The multi-subunit Type III-A CRISPR-Cas effector complex (Csm) exemplifies this principle and is in addition regulated by cellular metabolites such as divalent metals and ATP. Recognition of the foreign or cognate target RNA (CTR) triggers its single-stranded deoxyribonuclease (DNase) and cyclic oligoadenylate (cOA) synthesis activities. The same activities remain dormant in the presence of the self or non-cognate target RNA (NTR) that differs from CTR only in its 3′-protospacer flanking sequence (3′-PFS). The single-stranded DNase (ssDNase) and the cOA synthesis activities reside within the Csm1 subunit and the RNase activity resides within Csm317–19.

In contrast, a target RNA that complements both the guide region and the 5′-tag of the crRNA (alternatively referred to as the non-cognate target RNA, or NTR) is unable to switch on the Csm1-mediated activities. The 3′-PFS of NTR differs from that of CTR-43 and bears a complementary sequence to that of the crRNA 5′ tag. Seven of the eight PFS nucleotides are observed and only four form base pairs with the 5′ tag. Nucleotide (-1)′ is flipped out by the thumb loop of Csm4 similar to those at the cleavage sites. Nucleotides (-2)′–(-5)′ base pair with nucleotides (2–5) of the 5′ tag and (-6)′–(-7)′ rest on a groove formed by the Lid loop of Csm4 and the LiP loop of LlCsm1. Though the Csm1-Csm4 interface further reduces from 1261 Å2 in the CTR-bound to 929 Å2 in the NTR-bound complex, LlCsm1 gains 433 Å2 interfaces with 3′-PFS that in turn bases pairs with the 5′ tag of crRNA. As a result, 3′-PFS establishes an extensive interface that stabilizes Csm1 onto Csm4 and crRNA. Given the close resemblance in Csm1 structure between the CTR- and the NTR-bound LlCsm and the large distance between the 3′-PFS binding site and the HD domain, the strikingly different enzymatic activities between the two may be accounted for by their different dynamic behaviors. The refined atomic displacement parameter, or the B factor, combined with the map-fitting quality score, Q score, provides an indication that the Csm1 subunit is less stable in the CTR- than in the NTR-bound complex.

> MDKINLVCGSLLHNIGKIIYRGTSERAKHSKLGGDFIKSFEQFRNTELTDCIRYHHAQEITSVKSNKEKNSLFYITYIADNISSGMDRRKDLEEGAEGFNWDKKVALGSVFNVLNEKEKGRQNYSYPFVARTRIKEEPLNFPTATQNQYTTSYYDGLITDMKTILQRLKPDKEHINSLLQMMESLWSYVPSSTDKNQLVDISLYDHSRTTAAIASAIYDYFQAENITDYQKELFDYNATEFYDKNAFLMMNFDMSGVQNFIYNISGSKALKSLRARSFYLDMLLEYISDNLLEKLELSRANILYVGGGHAYLLLANTNKTKAILSDFEHDLKTWFLDKFKIDLYVAMAYTEVSANDLMNHNGHYRDIYRRLSQKTSAKKANRYTAEEILNLNHQGTENARECRECKRSDLLIEEDDICEICDSLQKVSRDLTRENIFVIANEGVLDMPFGKKMSALSYSQADKLKKSNAEVQIYAKNISEIGQNLMTRIDMGDYTYRSDFHEMLEEVEVGINRLGVLRADVDNLGQAFINGIPDDYLSISRTATFSRAMSRFFKNYLNQLLAEKSYKINVIYAGGDDLFMIGAWQDILDFSIVLKQKFADFTQNKLSISAGIGMFREKYPVARMASLTGDLEDAAKDYKPDERAVQATKNAVTLFDATNVFSWDTLENDIFVKLDAITKNFEKLDETGKAFIYRLIDLLRGVNENQQINIARLAYTLSRMEEKIGKTFAQELYNWANADRKTLIMALEIYILKTRE;> MKIIKLYFESPVHFGEKRLSESKITFSADTLFSALMIEAVGLGKEDEFYQLASNNLVKFSDAFPFIDQYYYIPKPMFNLKLEKEDENPSKAFKKLLYVPIDSLEDYLSGGLDAYFERESFNLGKLALSEKVQQHDFKDSEPYNVGTFTFKENTGLYVLIEQTHPLLEELLENLQYSGIGGKRNSGYGKFKFEILEDSDIEDLFSAKGNRKILLSGALPKDAELEQALKNASYLLERRGGFVQSDTYATNLVKKQDLYVFKSGSTFENSFDGDIYQVGKKGNHPVYKYAKSFFLEVSV;>TELKIGNEKVNSTNFGDFAEKAIRGINHKPFVNSKGGEQKITTSKIRGILELVNKVYNRVINTNDVELSENILADIAYIKVKIAYESGREPVVKDFIQRTAFTAAITDVMNQRTRESFLLFARYVESLIAYFKFYGGKD[3x];>MKLVIEGTIVLKTGMHIGGSSDFSAIGAVASPVVRDTLTRLPLIPGSSLKGKMRYLLAKELNNGILLNEPNNDQDEILRLFGSSEKDKIRRARLKFNDIKLSNLAELETFNVSSTEVKFENTINRKTAVANPRQIERVIAGSKFDFEIFYNLDDIKEVEKDFENIKQGFDLLEFDYLGGHGTRGSGRIAFENLSVITAVGNFEKINTLNEILGA[4x];> MKKTYRVTLTALGPIFIGGGEKLKKYEYIFDKQKKVAHMIDHTKFTKYLLEKNLLDDFTSRVNSHFDLYDYLVNKKGIVFMPLVKYSVPVAQFRTEVKNRFGKPISSPPMNDLNTFVKDAFGRPYIPGSSLKGALRTAILNDLKEDTKENEVFAHLQVSDSETIDLENLKVYQKVDYSKTAKPLPLYRECLKPNTEITFTVSFDDEYLTLKKIQNALHKTYQHYYIKWLKGGKVGETLIKGVYDSHADELKKNTFALDQPSQNQGEIIYIGGGAGFVSKTLHYKSKNRDQARNDSFDILKQLFRTTYSKMRSVPDNVPVALKLAVETKTFNGRVTGKHYLEMGKARIKLEEL> KIHTSYDEQSSGESKVKKIEFSKFTVKIKNKDKSGNWTDLGDLVVRKEENGIDTGLNAGGHSATFFSLEEEVVNNFVKVMTEGGSFKTSLYYGYKEEQSVINGIQNKEIITKIEKIDGTEYITFSGDKIKNSGDKVAEYAISLEELKKNLK;> KDSTGKCGPPPPIDNGGITSFPLSVYAPASSVEYQCANLYQLEGNKRITCRNGQWSEPPKCLHPCVISREIMENYNIALRWTAKQKLYSRTGESVEFVCKRGYRLSSRS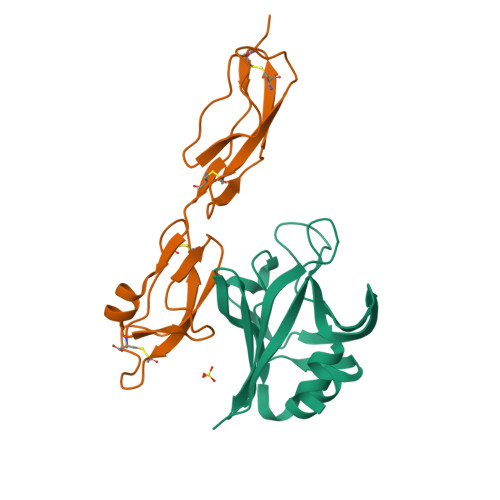HTLRTTCWDGKLEYPTCAKR Tailed bacteriophages and herpesviruses use a transient scaffold to assemble icosahedral capsids with hexameric capsomers on the faces and pentameric capsomers at all but one vertex where a 12-fold portal is thought to nucleate the assembly. We have determined the portal vertex structure of the bacteriophage HK97 procapsid, where the scaffold is a domain of the major capsid protein. Assembly of this large complex from hundreds of protein subunits requires transient association of an internal scaffolding protein or domain that acts similar to a chaperone and is absent from the mature capsid. The mcp gene 5 encodes a 103-residue N-terminal scaffolding domain (mcpN) and a 281-residue C-terminal domain (mcpC) that exhibits the HK97-fold including a triangular A-domain; a P-domain, composed of a long spine α helix; an adjacent three-stranded β sheet; the flexible E-loop; and the N-arm.

An initial map with icosahedral symmetry imposed was solved to 3.6-Å resolution for exploring the global organization of the Prohead. Our focused reconstruction of the penton vertices had sufficiently detailed side chain density to build a 30-residue model into the spokes (inset), which are composed of residues 76 to 103 of mcpN. This segment of scaffolding domain adopts a helix-turn-strand motif with residues S76 to S88 forming a rigid α helix lining the interior surface of the capsomer subunits, followed by a turn, and residues K92 to G97 adding an additional strand to the three-strand β sheet of the mcpC P-domain. The final model reveals that the density is discontinuous between residues L105 and R130, showing that the N-arm region is flexible. Hence, compared to Prohead II, the N-arm is not visible and the cleavage site, K103/S104, lies in a rather unstructured part of the shell. Our higher-resolution cryo-EM map of Prohead I shows notable differences with Prohead II, including visualization of ~25 mcpN residues bound to mcpC, displacement of one end of the spine helix, reorganization of the P-loops, and a complete absence of N-arm density. Our data show not only that the Prohead I P-domain is constrained (the spine helices are bent and even displaced from their positions in Prohead II) but also that the P-loops at the end of that domain adopt an arch conformation, preventing interaction with neighboring capsomers at the pseudo-threefold interfaces. At the icosahedral threefold, the P-loops interact closely with each other, but in a manner different than in Prohead II, probably because they align with the long axis of the Prohead I hexamer skew axis. The scaffold C terminus binds to both the spine helix and to the P-domain β sheet, which suggests a potential regulatory mechanism of assembly where the scaffolding domain locks the mcps of assembling capsomers into the Prohead conformation, thus constraining interactions between capsomers to specific sites that guide correct assembly and shell closure.

>MSELALIQKAIEESQQKMTQLFDAQKAEIESTGQVSKQLQSDLMKVQEELTKSGTRLFDLEQKLASGAENPGEKKSFSERAAEELIKSWDGKQGTFGAKTFNKSLGSDADSAGSLIQPMQIPGIIMPGLRRLTIRDLLAQGRTSSNALEYVREEVFTNNADVVAEKALKPESDITFSKQTANVKTIAHWVQASRQVMDDAPMLQSYINNRLMYGLALKEEGQLLNGDGTGDNLEGLNKVATAYDTSLNATGDTRADIIAHAIYQVTESEFSASGIVLNPRDWHNIALLKDNEGRYIFGGPQAFTSNIMWGLPVVPTKAQAAGTFTVGGFDMASQVWDRMDATVEVSREDRDNFVKNMLTILCEERLALAHYRPTAIIKGTFSSGS[7x]> MAGAQDFVPHTADLAELAAAAGECRGCGLYRDATQAVFGAGGRSARIMMIGEQPGDKEDLAGLPFVGPAGRLLDRALEAADIDRDALYVTNAVKHFKFTRAAGGKRRISKTPSRTEVVACRPWLIAEMTSVEPDVVVLLGATAAKALLGNDFRVTQHRGEVLHVDDVPGDPALVATVHPSSLLRGPKEERESA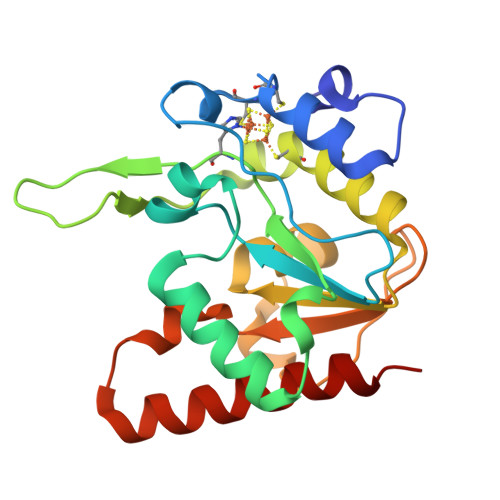FAGLVDDLRVAADVRP> MDIAKWVEHARTCYSTQLDTKIKVIGVIGKDYPDHGKGDNINCYLRENVFPVAATEDETCTIRGHFSEDDQILFLVMNGVDDVANIRKCLKSNPKSNYFDAMAESECQQIRMLHFLFISCHFIIIFEQTSRIDLELMRFLKKVNSARIQLRKKINQRLVASDLRDVSFNNRILSSAESEGRMVVPRLLIAFQRNNIRPDVNPGKKLQR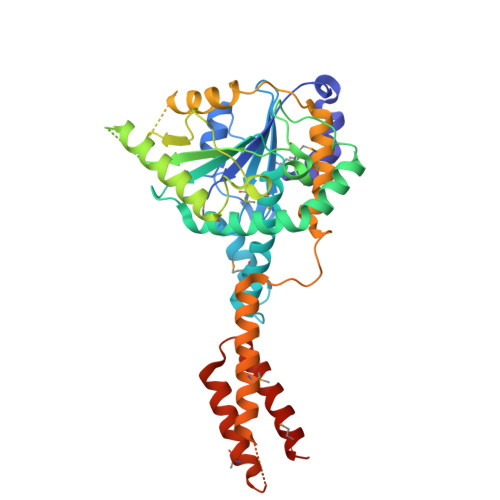ELYEKLEKNLDNQFSDILKLYDLIDCGASSLCQLNETIPVVHLLNPKIVKRDIIGEMFEILMADAENTKISGNAGTLPSNNSFVKFLEDNFRSEKNEISLENVIELMNCLQCVLDGDLEEKHEKTAIQTFIKRIQNDHMEEARRLYTNAQRPGERRGADRFKDSEKPVKIRSKEEHLMRFNEATHYIDSVVGVNSREALSQLQAQCNEMWQSDMRHHHHHH>SACKETGWPFCSDEDWNTKCPSGCRMKGLI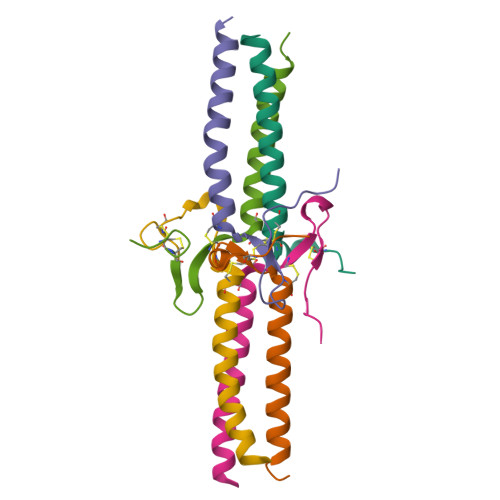DEVDQDFTSRINKLRDSLFNYQK[2x];>[2x]KVERKPPDADGCLHADPDLGVLCPTGCKLQDTLVRQERPIRKSIEDLRNTVDSVSR;>[2x]YVATRDNCCILDERFGSYCPTTCGIADFLNNYQTSVDKDLRTLEGILY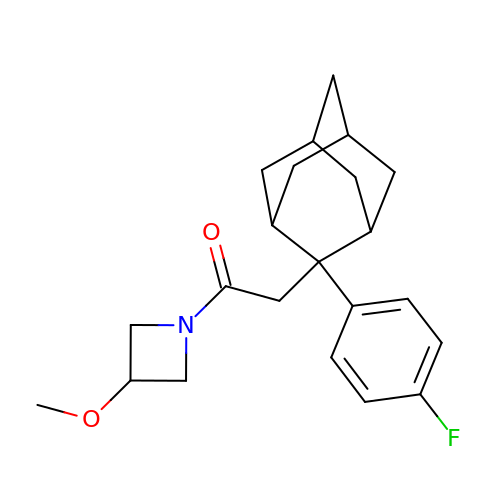2-[2-(4-fluorophenyl)-2-adamantyl]-1-(3-methoxyazetidin-1-yl)ethanone  | C22 H28 F N O2 | WUEWLMUHOBWRQF-BPYUXQLRSA-N>GPLGSHRHNELERERRFDMVVRVLARNISERMYTFEHGLRGARGA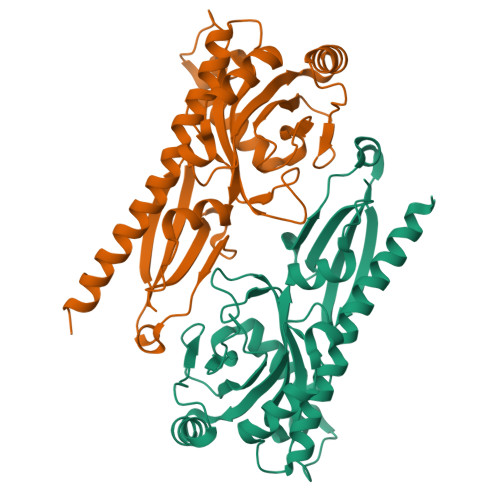VIGAGSDVISRDRFTRYSRSRDYPREFPGVLGYGYIHRVAAADEAAFLDAARADGAPDIQRRLLAPWDGERFIVLYFEPESSGNRPLGLDVASEPRRRIAAIAAARSGQPTMTSPVSLSGYQTPSEGGFLVLLPVYREGMPLQTPQQRMDATTGWAYAPLSVKQMLESTLGDRDDVAISLSDREDTQHTFYRSGIAAPESMRRAAHTQLLPIYGRTWVLTARPT[2x]>[2x]MMSETAPLPSASSALEDKAASAPVVGI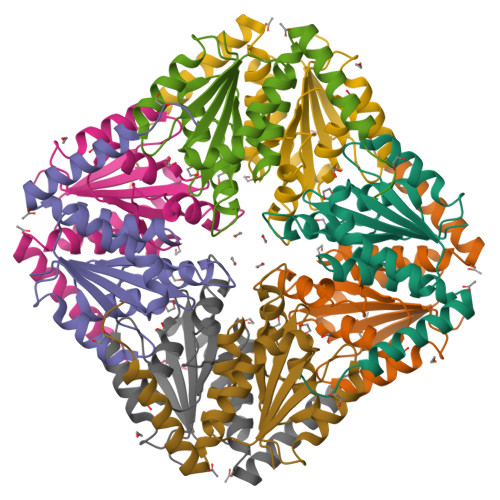IMGSQSDWETMRHADALLTELEIPHETLIVTAHRTPDRLADYARTAAERGLNVIIAGAGGAAHLPGMCAAWTRLPVLGVPVESRALKGMDSLLSIVQMPGGVPVGTLAIGASGAKNAALLAASILALYNPALAARLETWRALQTASVPNSPITEDK>[4x]SHVEYSRITKFFQEQPLEGYTLFSHRSAPN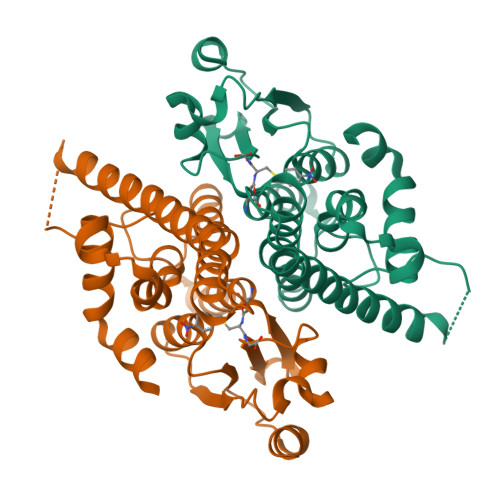GFKVAIVLSELGFHYNTIFLDFNLGEHRAPEFVSVNPNARVPALIDHGMDNLSIWESGAILLHLVNKYYKETGNPLLWSDDLADQSQINAWLFFQTSGHAPMIGQALHFRYFHSQKIASAVERYTDEVRRVYGVVEMALAERREALVMELDTENAAAYSAGTTPMSQSRFFDYPVWLVGDKLTIADLAFVPWNNVVDRIGINIKIEFPEVYKWTKHMMRRPAVIKALRGE BthA is the first example of a diheme enzyme carrying out chemistry reminiscent of both canonical bCCPs and MauG. Our efforts reveal that BthA is a peroxidase, capable of both H2O2 turnover when in the presence of an external electron source, yet also generates the bis-Fe(IV) species, as determined by Near-infrared  (NIR) and Mössbauer spectroscopy. Surprisingly, the kinetic parameters of H2O2 turnover indicate BthA is a very good peroxidase despite its spectroscopic and electrochemical parallels to MauG. BthA is also capable of generating the putative bis-Fe(IV) species and produces an electronic absorption spectrum similar to peroxide-treated MauG.

The structure of BthA was solved using X-ray crystallography to 1.54-Å resolution, revealing the same overall fold found in other structurally characterized bCCPs and MauG. The 6c heme pocket in BthA is more similar to MauG, showing Tyr-His ligation by Tyr463 and His 371. In place of this interheme tryptophan residue, BthA has a serine residue, Ser257. Importantly, both S257A and S257W variants generated the bis-Fe(IV) species based on detection of the 960 nm feature in NIR and yielded nearly identical kinetic values for peroxide turnover. A final trait common to MauG and bCCPs is a catalytically essential Ca2+ ion located between the propionate moieties of the two hemes. In place of a calcium ligand, BthA contains a lysine residue, Lys444, which mediates a similar solvent network between the heme cofactors. However in the BthA structure, the ε-ammonium group of Lys444 occupies the position of the conserved Ca2+ ion, one of the notable differences between BthA and MauG, suggesting that the positively charged Lys side-chain mimics a Ca2+ ion. Notably, the crystal structure revealed the presence of a unique surface-exposed disulfide bond between residues Cys415 and Cys430.

> ASSGPAAPDATHSTHAARPASAASSTSPMNPTSTPGASGPAHAKAALDAARAKAAPPSPPTTVLLPGAPPERVVDTIGRGTPQVASKVDPTAAVFRPDPTLAALGKRVFFDPALSEPRGMSCASCHDPGRAFAPTLSPAALAGPRVPQGSRPGHFSRRNAPSLLYVRYVPRRHFYQDDDALAPAPFGGLFSDGRADTLAEQLRGPLFDPDEMNNASAAALMRKIGRTGLGAALAGRFGPSVRRDPERMVRVLGEAMQAYLQSDEMAPFSSRYDAYVTKRAPLTPQEMRGLALFRNPDKGNCMSCHTLSDTASRPERSLFTDFGYDAIAVPRNRALPANRDPRHFDNGLCDTAAKLRWPEPTQWCAYLRTPGLRNVAIKESFMHNGVFDTLRDAVAFYNTRSTDPARWYHGRDTFDDVPRAYRGNVNVNSTPMNRRPGTPPAMTDADVDDLVAFLRTLTDARYVGLMPTAPDGKAARP> SVPKTGDSLAMARRLARSVRRLTRRRAHRLLRTRRLLKREGVLQAA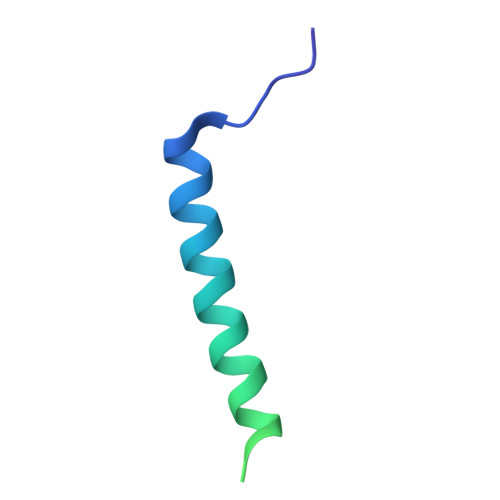NFDENGLIKSLPNTPWQLRAAALDRKLT>MAFELPNLPYGFRALEPHIDQQTMEIHHDKHHNTYVTKLNAAVEGTDLESKSIEEIVANLDSVPENIQTAVRNNGGGHLNHSLFWELLTPNSEEKGTVVDKIKEQWGSLDAFKEEFANQAAARFGCG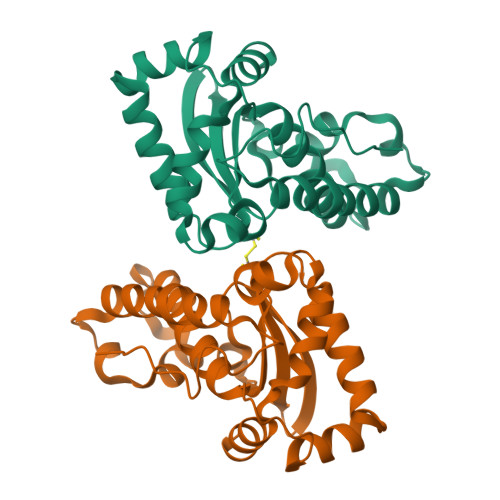WAWLVVNDGKLEIVTTPNQDNPLTEGKTPILGLDVWEHAYYLKYQNKRPDYISAFWNVVNWEKVDELYNAAKHHHHHH[6x]> GEIEFIESSKDAGFPVINTPSKTKLEPSVFHQVFEGNKEPAVLRSGDPRLKANFEEAIFSKYIGNVNTHVDEYMLEAVDHYAGQLATLDISTEPMKLEDAVYGTEGLEALDLTTSAGYPYVALGIKKRDILSKKTKDLTKLKECMDKYGLNLPMVTYVKDELRSIEKVAKGKSRLIEASSLNDS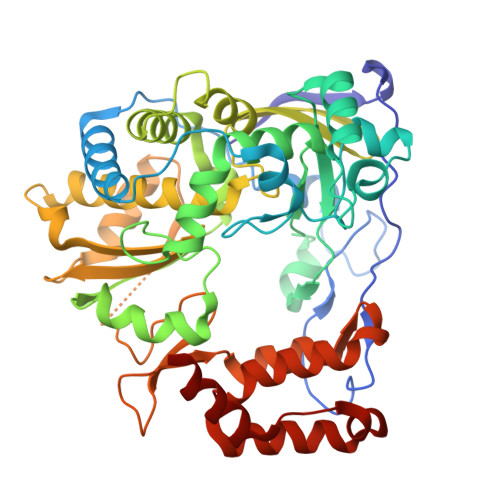VAMRQTFGNLYKTFHLNPGVVTGSAVGCDPDLFWSKIPVMLDGHLIAFDYSGYDASLSPVWFACLKMILEKLGYTHKETNYIDYLCNSHHLYRDKHYFVRGGMPSGCSGTSIFNSMINNIIIRTLMLKVYKGIDLDQFRMIAYGDDVIASYPWPIDASLLAEAGKGYGLIMTPADKGECLNEVTWTNVTFLKRYFRADEQYPFLVHPVMPMKDIHESIRWTKDPKNTQDHVRSLCLLAWHNGEHEYEEFIRKIRSVPVGRCLTLPAFSTLRRKWLDSF>GSDIPEHWEEDASWGPHRLAVLVPFRERFEELLVFVPHMRRFLSRKK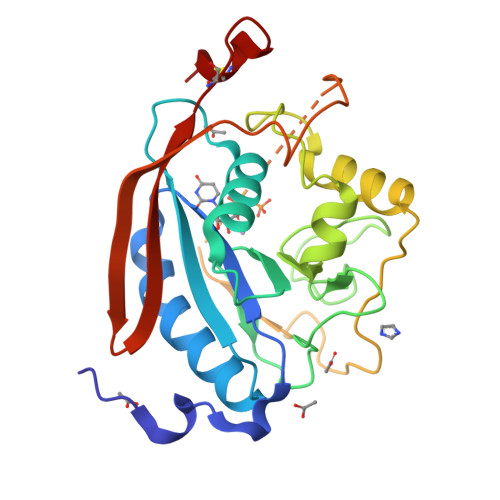IRHHIYVLNQVDHFRFNRAALINVGFLESSNSTDYIAMHDVDLLPLNEELDYGFPEAGPFHVASPELHPLYHYKTYVGGILLLSKQHYRLCNGMSNRFWGWGREDDEFYRRIKGAGLQLFRPSGITTGYKTFRHLHDPAWRKRDQKRIAAQKQEQFKVDREGGLNTVKYHVASRTALSVGGAPCTVLNIMLDCDKTATPWCTFS[2x]4,6-dideoxy-4-{[(1S,4R,5R,6S)-4-{[alpha-D-glucopyranosyl-(1->4)-alpha-D-glucopyranosyl-(1->4)-alpha-D-glucopyranosyl]oxy}-5,6-dihydroxy-3-(hydroxymethyl)cyclohex-2-en-1-yl]amino}-alpha-D-glucopyranose 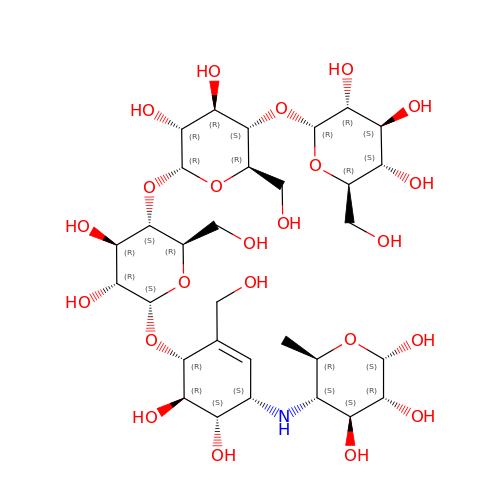| C31 H53 N O23 | SPMGVWYYOZMEBD-NPPSNIQKSA-N N-{(1S)-1-[5-(2-methoxyquinolin-3-yl)-1H-imidazol-2-yl]pentyl}-1-methylazetidine-3-carboxamide | C23 H29 N5 O2 | 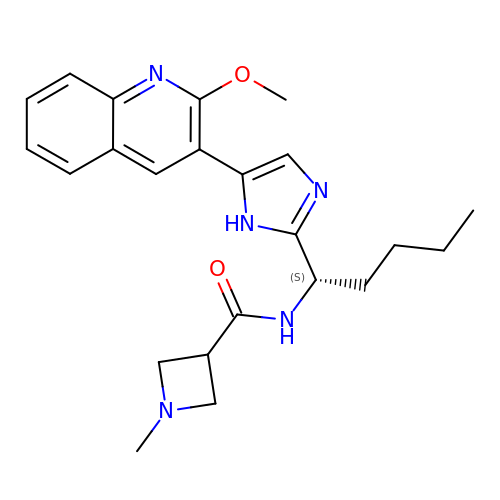AGQQCTCTRABOKI-IBGZPJMESA-N> AAEFWNEYEDFRSFFKKKFGKDLTGYQRLWAKRIVQGKSFTMVAPTGVGKTTFGMMTALWLARKGKKSALVFPTVTLVKQTLERLQKLADEKVKIFGFYSSMKKEEKEKFEKSFEEDDYHILVFSTQFVSKNREKLSQKRFDFVFVDDVDAVLKASRNIDTLLMMVGIPEEIIRKAFSTIKQGKIYERPKNLKPGILVVSSATAKPRGIRPLLFRDLLNFTVGRLVSVARNITHVRISSRSKEKLVELLEIFRDGILIFAQTEEEGKELYEYLKRFKF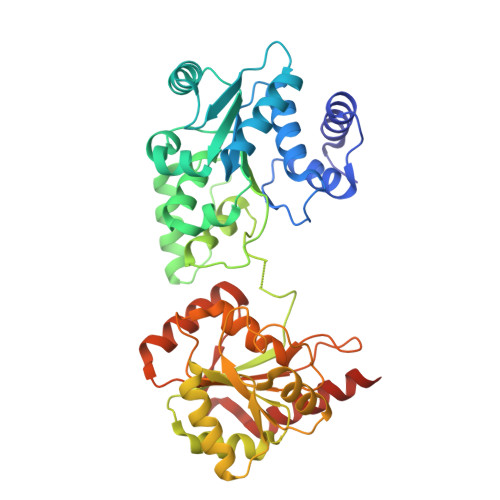NVGETWSEFEKNFEDFKVGKINILIGVQAYYGKLTRGVDLPERIKYVIFWGTPSGPDVYTYIQASGRSSRILNGVLVKGVSVIFEEDEEIFESLKTRLLLIAEEEIIEEAEANWKELVHEVEESRRRSERELTDTSR>[2x]SLTTTEVVMENVTAFWEEGGTPVLKDINFKIERGQLLAVAGSTGAGKTSLLMMIMGELEPSEGKIKHSGRISFCSQFSWIMPGTIKENIIGVSYDEYRYRSVIKACQLEED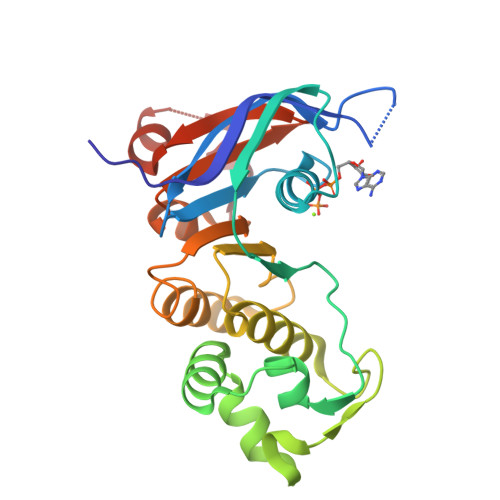ISKFAEKDNIVLGEGGITLSGGQRARISLARAVYKDADLYLLDSPFGYLDVLTEKEIFESCVCKLMANKTRILVTSKMEHLKKADKILILHEGSSYFYGTFSELQNLQPDFSSKLMG>[4x]MSTNEGSLWGGRFAGGPSDALAALSKSTHFDWVLAPYDLTASRAHTMVLFRAGLLTEEQRDGLLAGLDSLAQDVADGSFGPLVTDEDVHAALE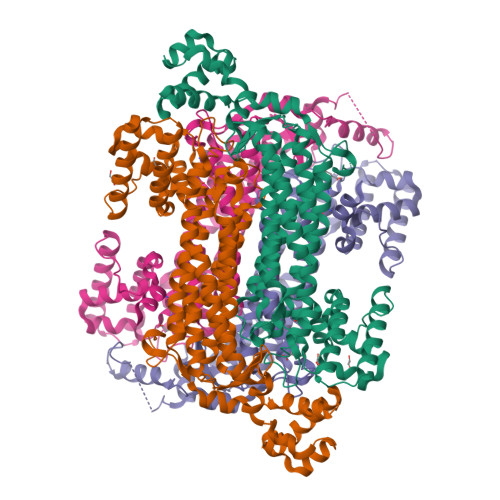RGLIDRVGPDLGGRLRAGRSRNDQVAALFRMWLRDAVRRVATGVLDVVGALAEQAAAHPSAIMPGKTHLQSAQPILLAHHLLAHAHPLLRDLDRIVDFDKRAAVSPYGSGALAGSSLGLDPDAIAADLGFSAAADNSVDATAARDFAAEAAFVFAMIAVDLSRLAEDIIVWSSTEFGYVTLHDSWSTGSSIMPQKKNPDIAELARGKSGRLIGNLAGLLATLKAQPLAYNRDLQEDKEPVFDSVAQLELLLPAMAGLVASLTFNVQRMAELAPAGYTLATDLAEWLVRQGVPFRSAHEAAGAAVRAAEQRGVGLQELTDDELAAISPELTPQVREVLTIEGSVSARDCRGGTAPGRVAEQLNAIGEAAERLRRQLVR> ETGICKG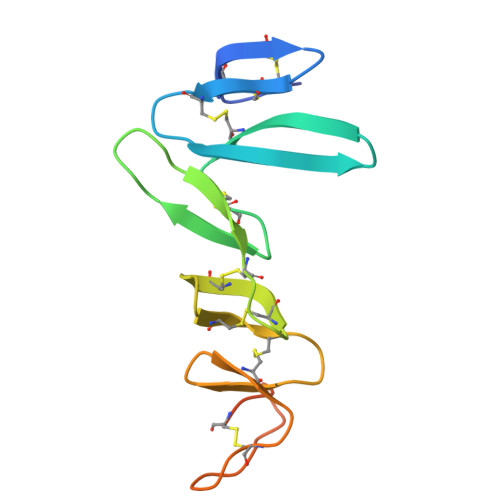CLSCSKDNGCSRCQQKLFFFLRREGMRQYGECLHSCPSGYYGHRAPDMNRCARCRIENCDSCFSKDFCTKCKVGFYLHRGRCFDECPDGFAPLDETMECVEGTHHHHHHHHHH>GGUGCGCC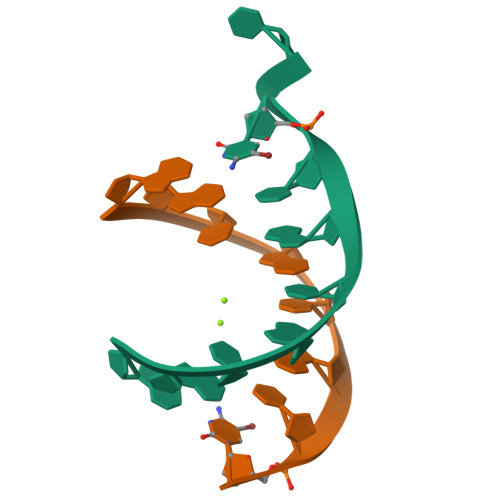C[2x]>MKKYRVQPDGRFELKRFDPDDTSAFEGGKQAALEALAVLNRRLEKLQELLYAEGQHKVLVVLQAMDAGGKDGTIRVVFDGVNPSGVRVASFGVPTEQELARDYLWRVHQQVPRKGELVIFDRSHYEDVLVVRVKNLVPQQVWQKRYRHIREFERMLADEGTTILKFFLHISKDEQRQRLQERLDNPEKRWKFRMGDLEDRRLWDRYQEAYEAAIRET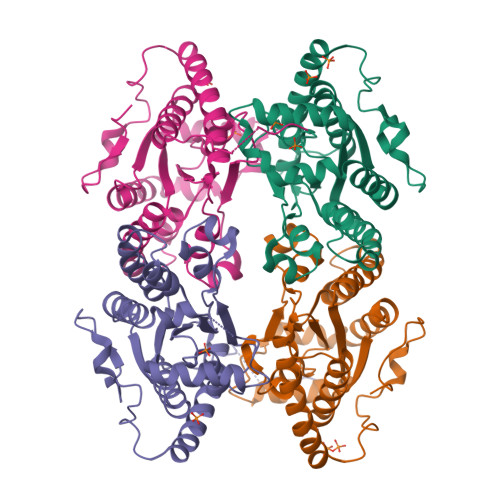STEYAPWYVIPANKNWYRNWLVSHILVETLEGLAMQYPQPETASEKIVIE[4x]4-(thiophen-2-yl)benzoic acid | C11 H8 O2 S | 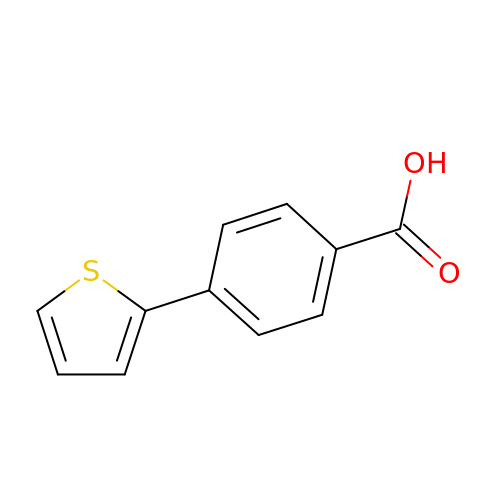CVDUBQJEQNRCIZ-UHFFFAOYSA-N> SSSQGLLGYYFSDLNFQAPMVVTSSTTGDLSIPSSELENIPSENQYFQSAIWSGFIKVKKSDEYTFATSADNHVTMWVDDQEVINKASNSNKIRLEKGRLYQIKIQYQRENPTEKGLDFKLYWTDSQNKKEVISSDNLQLPELKQKSSNSRKKRSTSAGPTVPDRDNDGIPDSLEVEGYTVDVKNKRTFLSPWISNIHEKKGLTKYKSSPEKWSTASDPYSDFEKVTGRIDKNVSPEARHPLVAAYPIVHVDMENIILSKNEDQSTQNTDSQTRTISKNTSTSRTHTSEVHGNAEVHASFFDIGGSVSAGFSNSNSSTVAIDHSLSLAGERTWAETMGLNTADTARLNANIRYVNTGTAPIYNVLPTTSLVLGKNQTLATIKAKENQLSQILAPNNYYPSKNLAPIALNAQDDFSSTPITMNYNQFLELEKTKQLRLDTDQVYGNIATYNFENGRVRVDTGSNWSEVLPQIQETTARIIFNGKDLNLVERRIAAVNPSDPLETTKPDMTLKEALKIAFGFNEPNGNLQYQGKDITEFDFNFDQQTLQNIKNQLAELNATNIYEVLDKIKLNAKMNILIRDKRFHYDRNNIAVGADESVVKEAHREVINSSTEGLLLNIDKDIRKILSGYIVEIEDTEGLKEVINDRYDMLNISSLRQDGKTFIDFKKYNDKLPLYISNPNYKVNVYAVTKENTIINPSENGDTSTNGIKKILIFSKKGYEIG

Protective antigen (PA) is an element of the protein toxin secreted by B. anthracis. It is a key component of recombinant Anthrax vaccines, since the immune response against this virulence factor confers protection against B. anthracis infection. The structure of PA reveals four domains. Domain 1 (grey) contains two calcium-binding sites and the furin cleavage site required for proteolytic activation of the molecule.

However, recombinantly PA (rPA) stored in aqueous solution is aggregation-prone. TANGO detects several APRs in the amino acid sequence of the protein. It was experimentally demonstrated that the solvent exposed APR (APR1) in domain 3 is the key determinant of rPA aggregation in vitro. Therefore, even though analysis suggests improvements are possible for all three APRs, we focused on APR1 (N573IYTVLD579). The MASS plot identified position Thr576 as a suitable design hot spot, allowing for mutation to Glu, Lys and Arg. An additional in silico mutation screen using FoldX revealed the stability of the T576E mutant could be improved by 1.2 kcal mol−1 by a compensatory mutation S559L. The mutant side chains were well defined in the electron density and superposed well with the predicted side-chain conformations by FoldX, further validating our approach. Far and near UV circular dichroism spectroscopy (CD) and near UV confirmed conservation of the structure between T576E/S559L and WT. Moveover, whereas WT shows characteristic signals of aggregation in the plot from 50 °C upwards, the T576E/S559L mutant starts aggregating only at a higher temperature, suggesting we have removed the APR responsible for aggregation during storage at room temperature. Plotting aggregation versus degree of unfolding, it appears the aggregation onset for WT occurs at 53% of the unfolding transition, whereas for the mutant aggregation only initiates at 84% of the unfolding transition. This is consistent with our design, in which we reduced the aggregation propensity of the strongest and most exposed APR by the T576E mutation, delaying aggregation until more advanced denaturation when the remaining APRs eventually become solvent exposed and initiate aggregation. Taken together, our data indicate that mutant T576E/S559L displays a lower aggregation propensity than the WT protein, while conservating both structure and biological activity of the PA protein.(3-(1H-tetrazol-5-yl)phenyl)boronic acid | C7 H7 B N4 O2 | 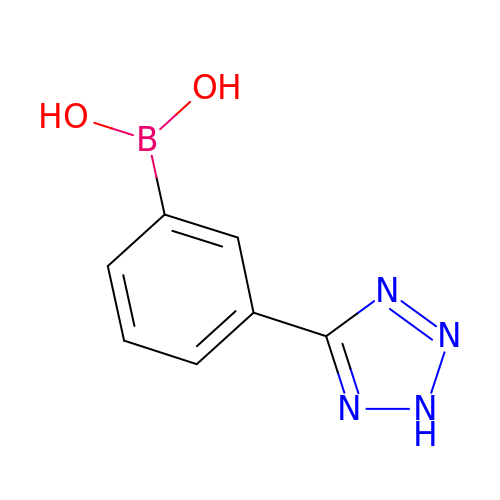XMJKBDSKRITXBW-UHFFFAOYSA-N5-methyl-7-propyl-1,6-naphthyridin-2(1H)-one | C12 H14 N2 O 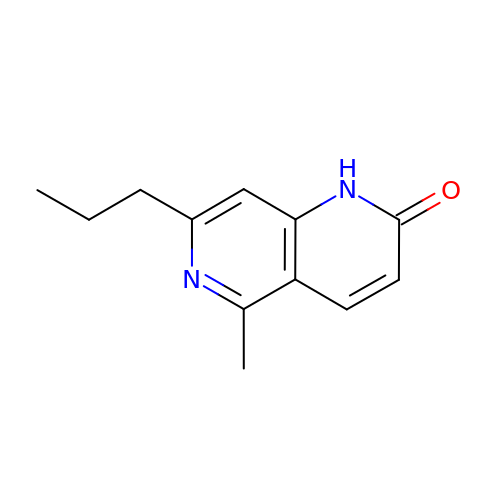| GNDSCMXBXGHCIV-UHFFFAOYSA-N>GPLSDLEVQPKPRPELDGPLPTVEELKEALEHGRLEVAWQVLALERQLEAAAAAGGMSNEELVWRQSKVEALYVLLCDQVLGVLRRPLEAAPERLSQALAVVSQEELEDRRASGGPLAAALEATRPRRWLQRWRGVVAEVAAERLDAQPATAPEGRSEAESRFLHMGRTMKEDLEVVVERLKPLFPDEFNVVRTYAESYHYHFASHLCALAQFELCERDTYLLLLWVQNLYPNDILNSPKLAQELQGVGLGSLLPPKQIRLLEAMFLSNEVTSVKQLMARALELESQRWTQDVAPQSLDGHCHSELAIDILQIISQGQTKAENITSDVGMQIKQLLLVELAALLRSYQRAFDEFLEKSKLLRNYRVNIMANINNCLFFWTSVEQKWQISHDSLNRLLEPLKDLKAHGFDTLLQSLFLDLKPLFKKFTQTRWANPVETLEEIITTVSSSLPEFSELQDCFREELMETVHLHLVKEYIIRLCKRRLVLKTAEQQQQLARHILANADAIQGFC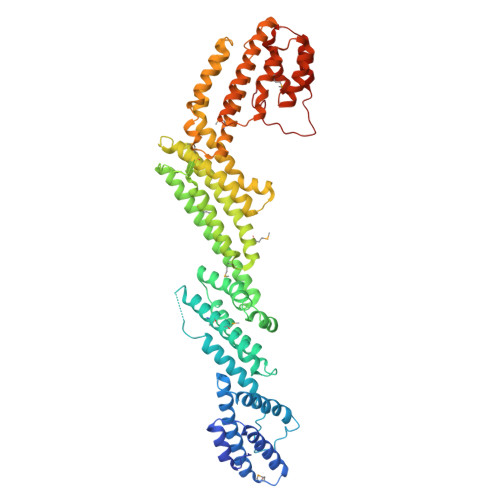TENGSTATWLHRALPMIAEIIRLQDSSAIKIEVATYATWYPDFSKGHLNAILAIKGNLPSSEVRSIRNILDINTGVQEPPRPLFSLIKVT[2x]>[4x]MHHHHHHLVPRGSEDELYRQ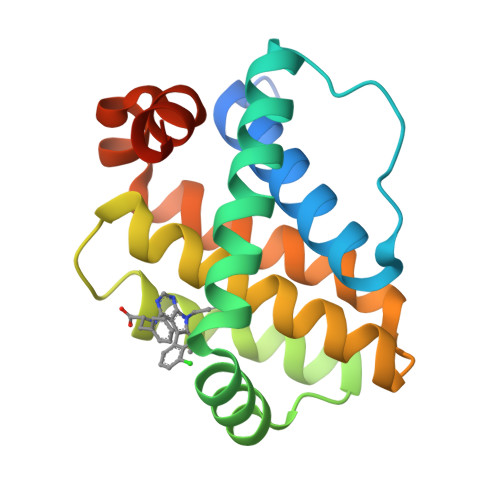SLEIISRYLREQATGAKDTKPMGRSGATSRKALETLRRVGDGVQRNHETAFQGMLRKLDIKNEDDVKSLSRVMIHVFSDGVTNWGRIVTLISFGAFVAKHLKTINQESCIEPLAESITDVLVRTKRDWLVKQRGWDGFVEFFHVEDLEGG> MAKPIEVTDQNFDETLGQHPLVLVDFWAEWCAPCRMIAPILEEIAKEYEGKLLVAKLDVDENPKTAMRYRVMSIPTVIL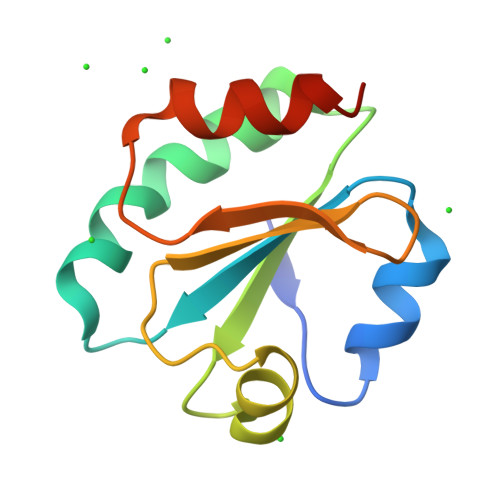FKDGQPVEVLVGAQPKRNYQAKIEKHLPATA> MSGIALSRLAQERKAWRKDHPFGFVAVPTKNPDGTMNLMNWECAIPGKKGTPWEGGLFKLRMLFKDDYPSSPPKCKFEPPLFHPNVYPSGTVCLSILEEDKDWRPAITIKQILLGIQELLNEPNIQDPAQAEAYTIYCQNRVEYEKRVRAQAKKFAPS;> NNDHINLKVAGQDGSVVQFKIKRHTPLSKLMKAYCERQGLSMRQIRFRFDGQPINETDTPAQLEMEDEDTIDVFQQQTGG;> SLTGEPAPVLSSPPPADVSTFLAFPSPEKLLRLGPKSSVLIAQQTD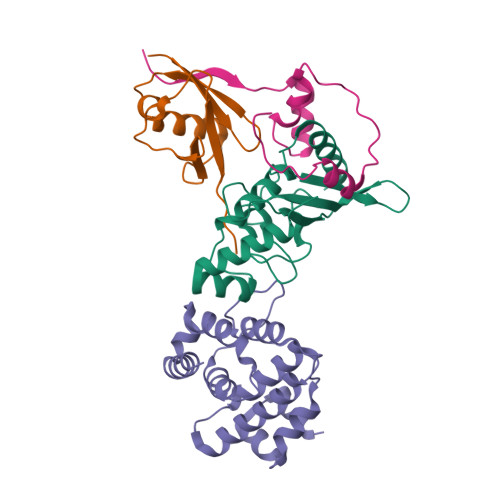TSDPEKVVSAFLKVSSVFKDEATVRMAVQDAVDALMQKAFNSSSFNSNTFLTRLLVHMGLLKSEDKVKAIANLYGPLMALNHMVQQDYFPKALAPLLLAFVTKPNSALESCSFARHSLLQTLYKV;> SLDDDVLIVYELTPTAEQKALATKLKLPPTFFCYKNRPDYVSEEEEDDEDFETAVKKLNGKLYLDGSEK> STENEKSRSLPAERNPLYKDDTLDHT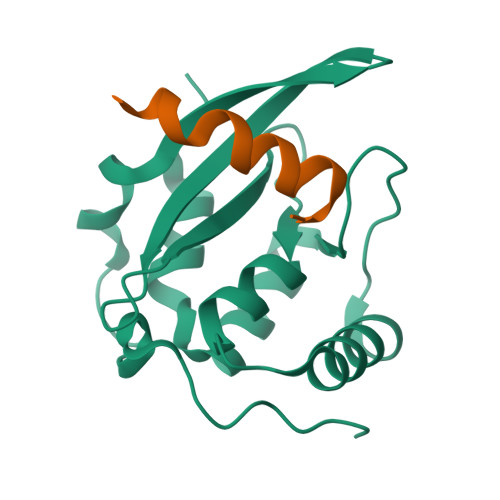PLIPKCRAQVIEFPDGPATFVRLKCTNPESKVPHFLMRMAKDSSISATSMFRSAFPKATQEEEDLEMRWIRDNLNPIEDKRVAGLWVPPADALALAKDYSMTPFINALLEASST;> GPLSDNEEFENVVKNGH>[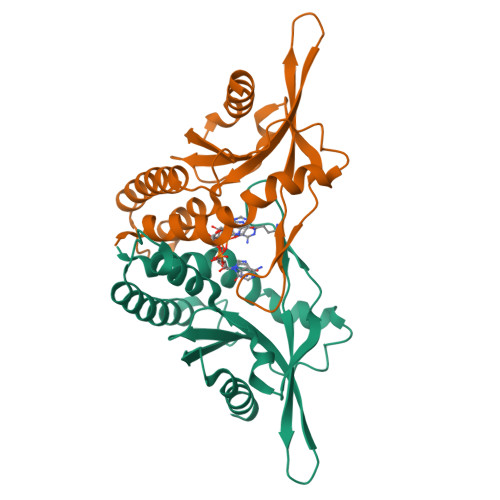2x]SNVADGLAWSYYFGYLRLVLPRLELRISESEYFRHKITDRKLFILLPKTCFTCDDIEQADSRVKWVGNLPESKINRGGIKERSYKHAVHEIVMPFPDGTEEKYHFIVEYATPLMSLYDMSRFTDAQLTGSERDHQVVLFIRKLTEILGKSEECKGRYELIPFSGDEDKNKIADILVALHNNANIMVDE>MGSVEEVKRIMDLARQKISDAMDELNMDATLKQSVDESMKRAEQRAYELSKTHEKTDALGQASADLARELVARNTSEDHQKQIFEALKKAAEEMAHRSDSHEDRLVMALILQTYANAKVTFRILNSGKALGKEDEAQKMADRWTRLSAEAASLSVQAINDSTSAEKMAENFRQAKE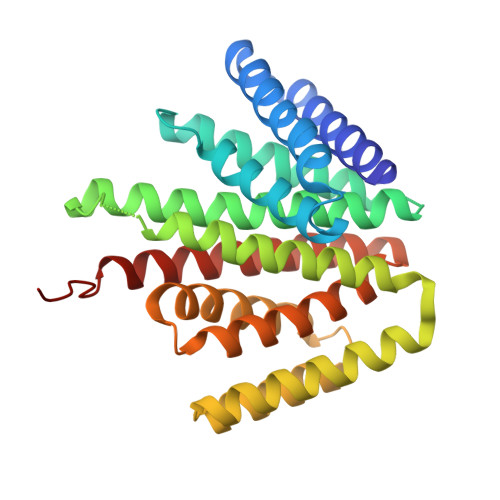DAVASLHRAGQDDLARKVSEFADAGLSKIDELMTLTGQMWAHGLFSKEWEDAARSLSRLAAVMLAQASQTKEGSLRAVKAMEKMADNAADEAEKLMKAGSENLYFQ[2x]>[2x]MAHHHHHHMHIHKIQAREILDSRGNPTIEADVTLTTGIIGRASVPSGASTGSREACELRDNDPKRYAGKGVQKAV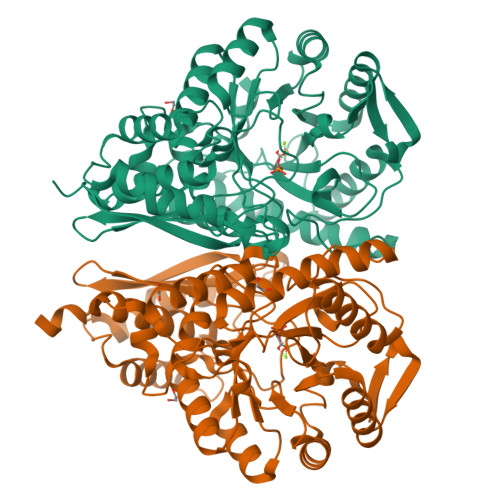KHVNNEINQALQGLSVEDQENLDRILCQLDNTENKSHLGANAILATSLACARARALSLNQPLYMTLNQGDMMTMPVPMMNILNGGAHADNNVDIQEFMIMPIGAPDFPVALQMGTEIFHVLKSVLKKQGLNTAVGDEGGFAPNIQSNRQALDLLSEAIEKAGFRLGEDIVFALDVAASELFNEGFYHMYSENQKFDSHQLIEYYANLISSYPIVSIEDGLDEKDWSGWKQLTTHLGNKVQLVGDDLFVTNPKILREGIAQGIANAILIKVNQIGTLSETRQAIKLAYDNGYRCVMSHRSGETEDTFIADLAVASGCGQIKTGSLCRTDRTAKYNQLLRINELASLPYAGKNILKR The T4BS secretion coupling complex of L. pneumophila comprises the inner membrane AAA+ ATPase DotL (IcmO) and two inner membrane/cytoplasmic components, DotM (IcmP) and DotN (IcmJ). In this study, we determine the crystal structure of the cytoplasmic domain of DotM and observe large patches of basic residues, leading us to hypothesize that DotM might form the recruiting platform for Glu-rich motif-containing effectors. Our results suggest that DotM’s cytoplasmic domain is capable of binding directly another subgroup of Legionella effectors that contain acidic Glu-rich motifs at their C terminus.

Further binding studies were conducted with several DotM mutants, where Arg residues (single or double) on the protein’s surface were mutated to Glu. Five mutants were produced: R196E/R197E (termed “M1”), R314E/R315E (termed “M2”), R347E/R348E (termed “M3”), R217E (termed “M4”), and R262E (termed “M5”). Binding was abrogated in M1, M2, and M4, indicating that these Arg patches are involved in binding of acidic Glu-rich peptides. To ascertain that the observed binding deficiency in M1, M2, and M4 variant proteins was not due to folding defects caused by the mutations, these three proteins were crystallized and their structures were determined and shown to be virtually identical to the wild-type protein. Thus, the mutations do not introduce structural defects, suggesting that the ITC binding results reflect an effective role of the residues in binding. The final model suggests that CegC3 is primarily helical. Binding is observed between the main middle Glu-rich helical motif of CegC3 (residues E155, E158, and E159; see numbering in Table 2 and interactions in Fig. 5) to the “central patch” residues R314 and R315, as well as between R217 of DotM to peptide residue E162. Remarkably (given that acidic Glu-rich motif-containing effectors represent only a subset of Legionella effectors), the M1 and M4 mutations resulted in a significant decrease in L. pneumophila replication in the macrophages (up to 70–80%). However, in A. castellanii, M1 reduces intracellular growth by up to 90% (after 24 h) while the slight reduction in intracellular growth of the M4 mutant is not statistically significant. We observed that the M1 and M4 dotM mutants producing the reporter fusions Cya-CegC3Cter, Cya-OSSCter, or Cya-Lpg1663Cter displayed lower levels of effector translocation compared to the wild-type strain of L. pneumophila (Cya-CegC3Cter: 50% and 30% decrease compared to wild-type DotM for M1 and M4, respectively; Cya-OSSCter: 50% and 40% decrease compared to wild-type DotM for M1 and M4, respectively; Cya-Lpg1663Cter: 60% and 55% decrease compared to wild-type DotM for M1 and M4, respectively).

>GPSGGGADVNKGPWAMALTPMEFARKYNLLRKDDALLDNPVPGEEMTAGIRRGDAKRVFTMQLGPYWDGFEECSPQAYALSAVFMARMNRDRDAANNILKVLDKTFVDGKPDFSVARPVMKKYQNSELVQEVVAKHAYVLTVIASLLEAAREDGVVPSSEFLWLKPVDRRLWYMLNCVGRQTPYSEVAGPFAHWKAEKEMGRRSLVPMIDEAIRALEIAVKEVRLTPRQMEELEP[2x]(2E)-3-{3-[(5-ETHYL-3-IODO-6-METHYL-2-OXO-1,2-DIHYDROPYRIDIN-4-YL)OXY]PHENYL}ACRYLONITRILE | C17 H15 I N2 O2 | 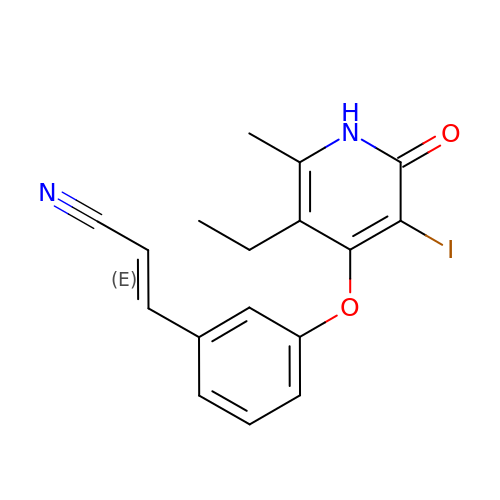XMFUXIRAVPMVRS-FNORWQNLSA-N> NTTGGRFVDKDNRKYYVKDDHKAIYWHK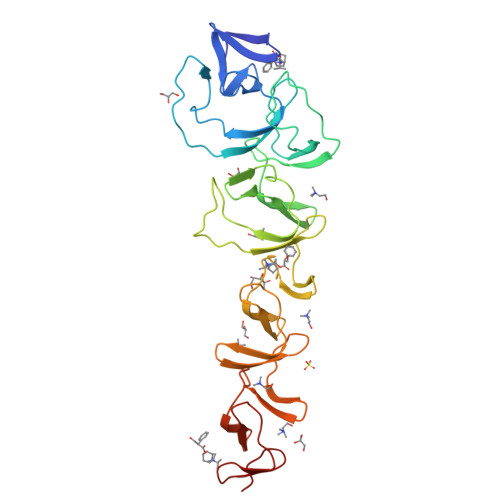IDGKTYYFGDIGEMVVGWQYLEIPGTGYRDNLFDNQPVNEIGLQEKWYYFGQDGALLEQTDKQVLEAKTSENTGKVYGEQYPLSAEKRTYYFDNNYAVKTGWIYEDGNWYYLNKLGNFGDDSYNPLPIGEVAKGWTQDFHVTIDIDRSKPAPWYYLDASGKMLTDWQKVNGKWYYFGSSGSMATGWKYVRGKWYYLDNKNGDMKTGWQYLGNKWYYLRSSGAMVTGWYQDGLTWYYLNAGNGDMKTGWFQVNGKWYYAYSSGALAVNTTVDGYSVNYNGEWVQ> MKFYIDDLPVLFPYPKIYPEQYNYMCDIKKTLDVGGNSILEMPSGTGKTVSLLSLTIAYQMHYPEHRKIIYCSRTMSEIEKALVELENLMDYRTKELGYQEDFRGLGLTSRKNLCLHPEVSKERKGTVVDEKCRRMTNGQAKRKLEEDPEANVELCEYHENLYNIEVEDYLPKGVFSFEKLLKYCEEKTLCPYFIVRRMISLCNIIIYSYHYLLDPKIAERVSNEVSKDSIVIFDEAHNIDNVCIESLSLDLTTDALRRATRGANALDERISEVRKVDSQKLQDEYEKLVQGLHSADILTDQEEPFVETPVLPQDLLTEAIPGNIRRAEHFVSFLKRLIEYLKTRMKVLHVISETPKSFLQHLKQLTFIERKPLRFCSERLSLLVRTLEVTEVEDFTALKDIATFATLISTYEEGFLLIIEPYEIENAAVPNPIMRFTCLDASIAIKPVFERFSSVIITSGTISPLDMYPRMLNFKTVLQKSYAMTLAKKSFLPMIITKGSDQVAISSRFEIRNDPSIVRNYGSMLVEFAKITPDGMVVFFPSYLYMESIVSMWQTMGILDEVWKHKLILVETPDAQETSLALETYRKACSNGRGAILLSVARGKVSEGIDFDHQYGRTVLMIGIPFQYTESRILKARLEFMRENYRIRENDFLSFDAMRHAAQCLGRVLRGKDDYGVMVLADRRFSRKRSQLPKWIAQGLSDADLNLSTDMAISNTKQFLRTMAQPTDPKDQEGVSVWSYEDLIKHQNSRKDQGGFIENENKEGEQDEDEDEDIEMQ;> MSHSGAAIFEKVSGIIAINEDVSPAELTWRSTDGDKVHTVVLSTIDKLQATPASSEKMMLRLIGKVDESKKRKDNEGNEVVPKPQRHMFSFNNRTVMDNIKMTLQQIISRYKDADIYEEKRRREESAQHTETPMSSSSVTAGTPTPHLDTPQLNNGAPLINTAKLDDSLSKEKLLTNLKLQQSLLKGNKVLMKVFQETVINAGLPPSEFWSTRIPLLRAFALSTSQKVGPYNVLSTIKPVASSENKVNVNLSREKILNIFENYPIVKKAYTDNVPKNFKEPEFWARFFSSKLFRKLRGEKIMQNDRGDVIIDRYLTLDQEFDRKDDDMLLHPVKKIIDLDGNIQDDPVVRGNRPDFTMQPGVDINGNSDGTVDILKGMNRLSEKMIMALKNEYSRTNLQNKSNITNDEEDEDNDERNELKIDDLNESYKTNYAIIHLKRNAHEKTTDNDAKSSADSIKNADLKVSNQQMLQQLSLVMDNLINKLDLNQVVPNNEVSNKINKRVITAIKINAKQAKHNNVNSALGSFVDNTSQANELEVKSTLPIDLLESCRMLHTTCCEFLKHFYIHFQSGEQKQASTVKKLYNHLKDCIEKLNELFQDVLN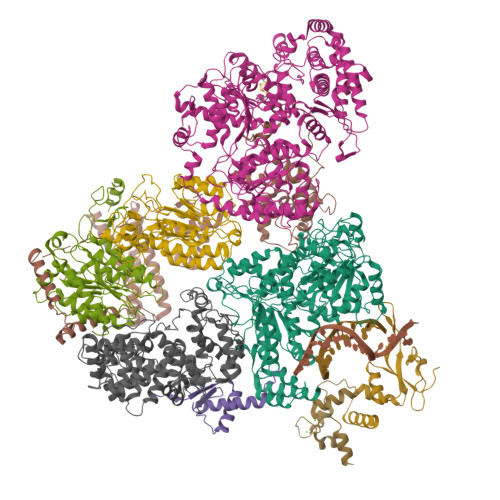GDGESMSNTCTAYLKPVLNSITLATHKYDEYFNEYNNNSN;> MSDYSLKHSVTQYLEEIPQQVQNRLYTSPATCLAIYRILPPLAKFFIMAMVFNENEVPLLDLDKWVNSNGKLQFQNAIKSMKSLHLLIPNKSSGTLMINLNPTFKISLRNALTGGEVQNSFGVVVEENVVSLDLLDEYSANKWETILHFMVGTPLAKIPSEKVLNLLKHSKLMEEVNSTGEFKITNEGFQFLLQEINSQLWTLLLQYLKMIETSKMDLVDVLHFIFMLGALEVGKAYKIDALSETQRIMLQDMRDYGLVFQKHSNDSIFYPTKLALMLTSDTKTIRSASNAMDSVLRQNREEPSVNEDGANGKSTTDITTSDDLNKAGLKNQDIPDGSLIVETNFKIYSYSNSPLQIAVLSLFVHLKARFVNMVLGQITRESIRRALTNGITADQIIAYLETHAHPQMRRLAEEKLEKKLELDPNCKEPLQVLPPTVVDQIRLWQLELDRVITYEGSLYSDFETSQEYNLLSKYAQDIGVLLWKDDKKKKFFISKEGNSQVLDFAKRKLKKKQ;> MDAISDPTFKHARSRKQVTEESPSLLTVIIEIAPKLWTTFDEEGNEKGSIIKVLEALIVFLNAHLAFNSANKVAVIAAYSQGIKYLYPESTSALKASESENKTRSDLKIINSDMYRRFRNVDETLVEEIYKLFELEKKQIEQNSQRSTLAGAMSAGLTYVNRISKESVTTSLKSRLLVLTCGSGSSKDEIFQYIPIMNCIFSATKMKCPIDVVKIGGSKESTFLQQTTDATNGVYLHVESTEGLIQYLATAMFIDPSLRPIIVKPNHGSVDFRTSCYLTGRVVAVGFICSVCLCVLSIIPPGNKCPACDSQFDEHVIAKLKRKPVVPRLKAKKKVTKP;> ARARKGALVQCDPSIKALILQIDAKMSDIVLEELDDTHLLVNPSKVEFVKHELNRLLSKNIYNPMD;> MAPVVISESEEDEDRVAITRRTKRQVHFDGEGDDRVDQQQQQHSSSHRDRDKHVQRKKKKRLSNRNLQGSNGGYAWEDEIKRSWDLVKVDDEGDMASLVASIVEARKKRTAKKNITPYQRGIIRSLILTLDCSEAMLEKDLRPNRHAMIIQYAIDFVHEFFDQNPISQMGIIIMRNGLAQLVSQVSGNPQDHIDALKSIRKQEPKGNPSLQNALEMARGLLLPVPAHCTREVLIVFGSLSTTDPGDIHQTIDSLVSEKIRVKVLGLSAQVAICKELCKATNYGDESFYKILLDETHLKELFNEAVTPLPVNKINKGFTLVKMGFPTRIFEDTPTFCSCHSKLVYGGYFCPNCHSKVCSLPTVCPCCDLMLILSTHLARSYHHLMPLKTFAEVPTTEKFRSEDCFSCQSRFPILKNHKNGKLLTSSRYRCEDCKQEFCVDCDVFIHEILHNCPGCESKPVIT;> MTDVEGYQPKSKGKIFPDMGESFFSSDEDSPATDAEIDENYDDNRETSEGRGERDTGAMVTGLKKPRKKTKSSRHTAADSSMNQMDAKDKALLQDTNSDIPADFVPDSVSGMFRSHDFSYLRLRPDHASRPLWISPSDGRIILESFSPLAEQAQDFLVTIAEPISRPSHIHEYKITAYSLYAAVSVGLETDDIISVLDRLSKVPVAESIINFIKGATISYGKVKLVIKHNRYFVETTQADILQMLLNDSVIGPLRIDSDHQVQPPEDVLQQQLQQTAGKPATNVNPNDVEAVFSAVIGGDNEREEEDDDIDAVHSFEIANESVEVVKKRCQEIDYPVLEEYDFRNDHRNPDLDIDLKPSTQIRPYQEKSLSKMFGNGRARSGIIVLPCGAGKTLVGITAACTIKKSVIVLCTSSVSVMQWRQQFLQWCTLQPENCAVFTSDNKEMFQTESGLVVSTYSMVANTRNRSHDSQKVMDFLTGREWGFIILDEVHVVPAAMFRRVVSTIAAHAKLGLTATLVREDDKIGDLNFLIGPKLYEANWMELSQKGHIANVQCAEVWCPMTAEFYQEYLRETARKRMLLYIMNPTKFQACQFLIQYHERRGDKIIVFSDNVYALQEYALKMGKPFIYGSTPQQERMNILQNFQYNDQINTIFLSKVGDTSIDLPEATCLIQISSHYGSRRQEAQRLGRILRAKRRNDEGFNAFFYSLVSKDTQEMYYSTKRQAFLVDQGYAFKVITHLHGMENIPNLAYASPRERRELLQEVLLKNEEAAGIEVGDDADNSVGRGSNGHKRFKSKAVRGEGSLSGLAGGEDMAYMEYSTNKNKELKEHHPLIRKMYYKNLKK;> MNEDLPKEYFELIRKALNEKEAEKAPLSRRRRVRRKNQPLPDAKKKFKTGLNELPRESVVTVNLDSSDDGVVTVPTDDSVEEIQSSEEDYDSEEFEDVTDGNEVAGVEDISVEIKPSSKRNSDARRTSRNVCSNEERKRRKYFHMLYLVCLMVHGFIRNEWINSKRLSRKLSNLVPEKVFELLHPQKDEELPLRSTRKLLDGLKKCMELWQKHWKITKKYDNVGLYMRTWKEIEMSANNKRKFKTLKRSDFLRAVSKGHGDPDISVQGFVAMLRACNVNARLIMSCQPPDFTNMKIDTSLNGNNAYKDMVKYPIFWCEVWDKFSKKWITVDPVNLKTIEQVRLHSKLAPKGVACCERNMLRYVIAYDRKYGCRDVTRRYAQWMNSKVRKRRITKDDFGEKWFRKVITALHHRKRTKIDDYEDQYFFQRDESEGIPDSVQDLKNHPYYVLEQDIKQTQIVKPGCKECGYLKVHGKVGKVLKVYAKRDIADLKSARQWYMNGRILKTGSRCKKVIKRTVGRPKGEAEEEDERLYSFEDTELYIPPLASASGEITKNTFGNIEVFAPTMIPGNCCLVENPVAIKAARFLGVEFAPAVTSFKFERGSTVKPVLSGIVVAKWLREAIETAIDGIEFIQEDDNRKEHLLGALESWNTLLLKLRIRSKLNSTYGKIAEEEPNVTKEQNIADNHDNTETFMGGGFLPGIANHEARPYSEPSEPEDSLDYVSVDKAEESATDDDVGEDYSDFMKELEMSEESD;> MSKSTNVSYERVELFENPKVPIEVEDEILEKYAESSLDHDMTVNELPRFFKDLQLEPTIWKLVRNEDVIIEGTDVIDFTKLVRCTCQLLILMNNLTVIDDLWSMLIRNCGRDVDFPQVALRDHVLSVKDLQKISNLIGADQSSGTIEMISCATDGKRLFMTYLDFGCVLGKLGYLKM> MIFSVDKVRADFPVLSREVNGLPLAYLDSAASAQKPSQVIDAEAEFYRHGYAAVHRGIHTLSAQATEKMENVRKR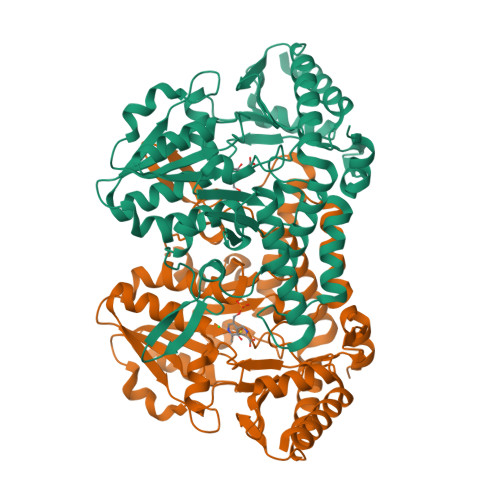ASLFINARSAEELVFVRGTTEGINLVANSWGNSNVRAGDNIIISQMEAHANIVPWQMLCARVGAELRVIPLNPDGTLQLETLPTLFDEKTRLLAITHVSNVLGTENPLAEMITLAHQHGAKVLVDGAQAVMHHPVDVQALDCDFYVFSGHKLYGPTGIGILYVKEALLQEMPPWEGGGSMIATVSLSEGTTWTKAPWRFEAGTPNTGGIIGLGAALEYVSALGLNNIAEYEQNLMHYALSQLESVPDLTLYGPQNRLGVIAFNLGKHHAYDVGSFLDNYGIAVRTGHHCAMPLMAYYNVPAMCRASLAMYNTHEEVDRLVTGLQRIHRLLG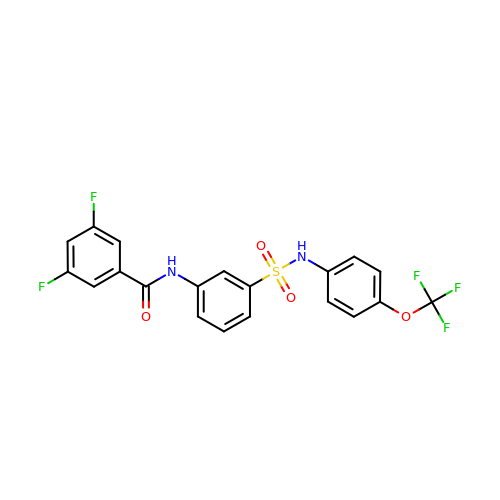3,5-bis(fluoranyl)-~{N}-[3-[[4-(trifluoromethyloxy)phenyl]sulfamoyl]phenyl]benzamide | C20 H13 F5 N2 O4 S | VSBQYLPAMTYZNU-UHFFFAOYSA-N>MISRIMLHKNTLLFAALSAALWGGATQAANAAVVASLKPLGFIASAIADGVTDTQVLLP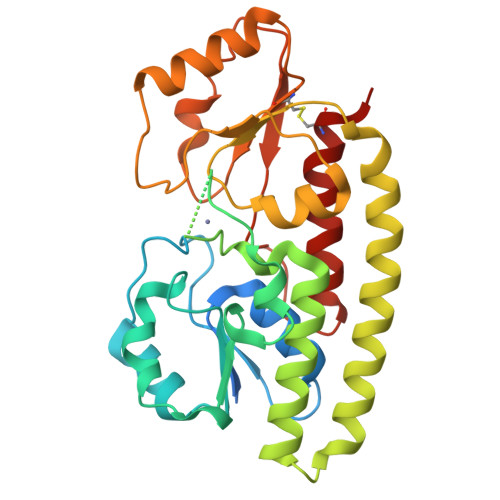DGASEHDYSLRPSDVKRLQGADLVVWIGPEMEAFMEKSVKNIPDGKQVTIAQLADVKPLLMKGADDDHDHGHEHGEKGDAHHHHGDYNMHLWLSPEIARASAVAIHEKLVELMPQSRAKLDANLKDFEAQLAATDKQVGNELAPLKGKGYFVFHDAYGYYEKHYGLTPLGHFTVNPEIQPGAQRLHEIRTQLVEQKATCVFAEPQFRPAVVEAVARGTSVRMGTLDPLGTNIKLGKTSYSAFLNQLANQYASCLKGD[6x]An L-arabinonate dehydratase from Rhizobium leguminosarum bv. trifolii catalyzes the rate-limiting step in the non-phosphorylative oxidative pathways, that is, converts sugar acid to 2-dehydro-3-deoxy sugar acid. A quaternary structure of RlArDHT is a homotetramer, and the active site is formed in the dimeric interface in a manner in which an N-terminal α-helix (particularly residues Arg22 − Trp30) and a C-terminus of one monomeric unit contribute to the formation of the active site of the partnering monomer. Each active site contains a [2Fe-2S] cluster and a magnesium ion. The last residue of the C-terminal tail, His579, participates in the formation of the substrate-binding cavity of the neighboring monomer.

To study the detailed effect of C-terminus mutation on the three-dimensional structure, the crystal structure of variant H579L with product analog 2-oxobutyrate was determined. Four polypeptide chains, or a tetramer, were observed in the asymmetric unit. In the H579L variant structure, this helix − loop − helix region was observed in the closed-form conformation. When the His residue is substituted for the Leu residue, the interaction with the Glu453 residue vanishes, and the side chain of Leu is rotated. The rotated Leu side chain also induces the conformational change of a nearby residue, Asp23, from the recognition helix. These subtle changes result in a larger substrate-binding cavity despite the almost interchangeable size of the residues His and Leu. 2-Oxobutyrate was refined inside the substrate-binding cavity in chain D of the H579L variant. The oxygen atom O1 of the carboxylate group at C1 position and the oxygen atom O3 of the carbonyl group at C2 of 2-oxobutyrate were both coordinated to the Mg2+. In addition to the 2-oxobutyrate ligand, the residues Glu91, Asp128, KCX129 (6N-carboxylysine), and Glu453 were coordinated to Mg2+, leading to octahedral coordination geometry. The distance between C3 of 2-oxobutyrate and Fe2 of the [2Fe-2S] cluster was 4.4 Å, which would leave sufficient space for the hydroxyl group of the substrate.

>[4x]MDWSHPQFEKKKKAEWPRKLRSQEWYGGTSRDVIYHRGWLKNQGYPHDLFDGRPVIGILNTWSDMTPCNGHLRELAEKVKAGVWEAGGFPLEVPVFSASENTFRPTAMMYRNLAALAVEEAIRGQPMDGCVLLVGCDKTTPSLLMGAASCDLPSIVVTGGPMLNGYFRGERVGSGTHLWKFSEMVKAGEMTQAEFLEAEASMSRSSGTCNTMGTASTMASMAEALGMALSGNAAIPGVDSRRKVMAQLTGRRIVQMVKDDLKPSEIMTKQAFENAIRTNAAIGGSTNAVIHLLAIAGRVGIDLSLDDWDRCGRDVPTIVNLMPSGKYLMEEFFYAGGLPVVLKRLGEAGLLHKDALTVSGETVWDEVKDVVNWNEDVILPAEKALTSSGGIVVLRGNLAPKGAVLKPSAASPHLLVHKGRAVVFEDIDDYKAKINDDNLDIDENCIMVMKNCGPKGYPGMAEVGNMGLPPKVLKKGILDMVRISDARMSGTAYGTVVLHTSPEAAVGGPLAVVKNGDMIELDVPNRRLHLDISDEELARRLAEWQPNHDLPTSGYAFLHQQHVEGADTGADLDFLKGCRGNAVGKDSL> MASSYSASAEP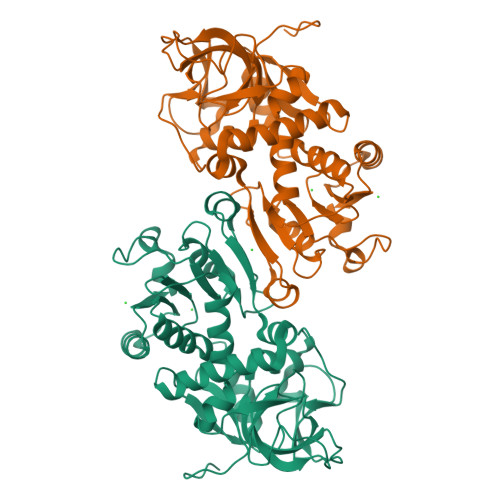ARVRALVYGHHGDPAKVVELKNLELAAVRGSDVRVKMLAAPINPSDINMIQGNYGLLPELPAVGGNEGVAQVVAVGSNVTGLKPGDWVIPANAGLGTWRTEAVFSEEALIQVPSDIPLQSAATLQVNPCTAYRMLMDFEQLQPGDSVIQNASNSGVGQAVIQIAAALGLRTINVVRDRPDIQKLSDRLKSLGAEHVITEEELRRPEMKNFFKDMPQPRLALNCVGGKSSTELLRQLARGGTMVTYGGMAKQPVVASVSLLIFKDLKLRGFWLSQWKKDHSPDQFKELILTLCDLIRRGQLTAPACSQVPLQDYQSALEASMKPFISSKQILTMLEHHHHHH> MVRKPVVSTISKGGYLQGNVNGRLPSLGSKEPPGQEKVQLKREITLLDGVSLIVGTIIGAGIFVSPKG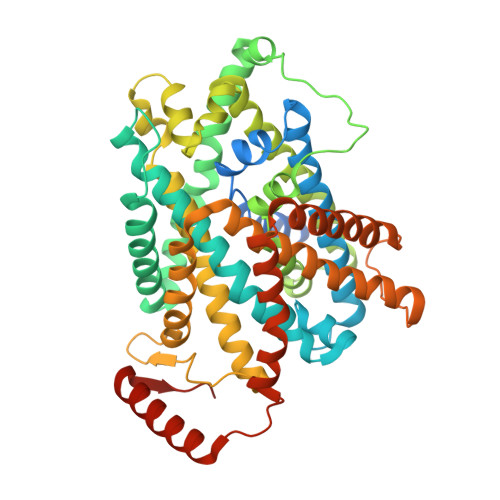VLKNTGSVGLSLVIWAVCGVLSLFGALCYAELGTTIPKSGGAYLYILETFGPLPAFLRGWNELLIIRPASTAVISLAFGNYILEPFFPTCEPPELAIKLLAAVGILLLTVLNSLSVKWSARVQDFFTAAKLLALLIIIVPGVVQLIKGQTQNFKDAFEGSDPSIGGLPLAFYSGLYAYVGWDYLNFVTEEVKNPEKNIPLAIVISMPIVTVAYVLTNVAYFTTLSPEELLLSNAVAVTFGERLLGNFSWAVPIFVALSCFGSLNGSLFAMSRLFYVAAREGHLPKILSMIHVRRHTPLPALIVSGPLTAIMLFLGDLFSLINFMSFGTWLFYGLVVAGLIYLRYKKPDLHRPIKVPLFIPILFLLTCLFLVAVSLYSDPVNCGIGFVIILTGVPVYFLFVYWDKKPKWFRRISEKITRHLQLLLEVVPEEDKLDYKDDDDK>[3x]QGNYLTANDVSKIRVGMTQQQVAYALGTPLMSDPFGTNTWFYVFRQQPGHE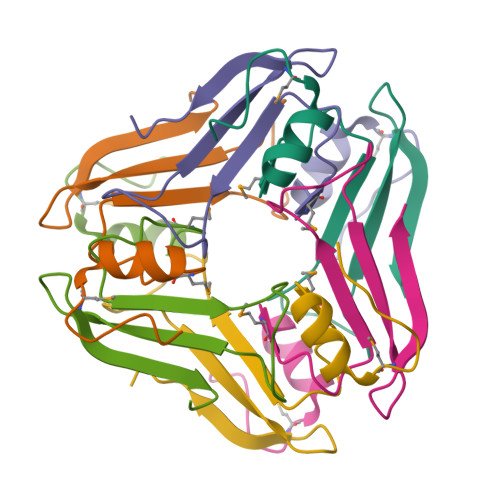GVTQQTLTLTFNSSGVLTNIDNKPALSGNLEHHHHHH> TTNTDSFTFSKFKPNQ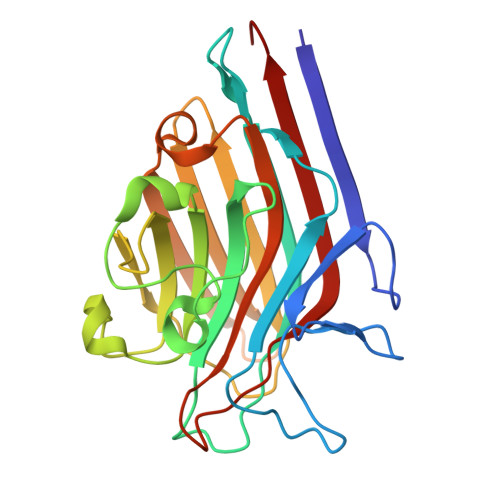PNLKKQGDATVTSSGTLQLTKVDKNGVPDPKSLGRALYASPINIWDSKTGVVASFATSFRFTIYAPNIATIADGLAFFLAPVSSPPKAGAGFLGLFDSAVFNSSYQTVAVEFDTYENTVFLDPPDTHIGIDVNSIKSIKTVKWDLANGEAAKVLITYDSSAKLLVAALVYPSSKTSFILSDVVDLKSVLPEWVSIGFSAATGASSGYIETHDVFSWSFASKLSFAA>[2x]GHMSTTARYDSIGGLFEDFTQSAAQRAIEVRTIFH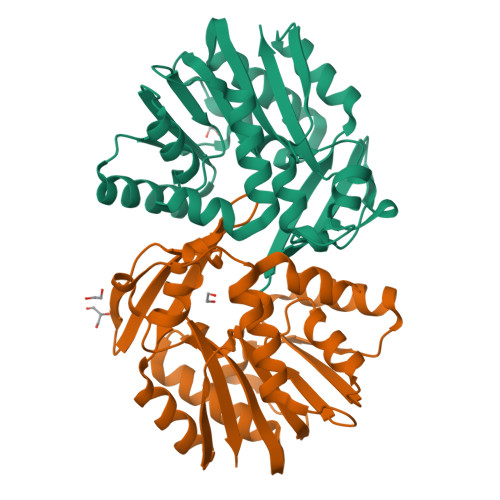MIGDVSGKSVLDLACGFGFFGREIYRRGAAKVVGVDISEKMIELAREESRKYGDPLEFHVRDVANMEPLGQFDLVNAAWLFNYADSVENLRKMFKVVRASLKPDGKLVAYTVDPDFSLAKGNFAKYGVNVLNERAWGPGYRHDAEFVTDPPSQFSFYRWSRADYESAIADAGFSHFEWQKPLLEADDIATHPPGFWDVFQNNCLQTGLVCKP> GSMKGSRIELGDVTPHNIKQLKRLNQVIFPVSYNDKFYKDVLEVGELAKLAYFNDI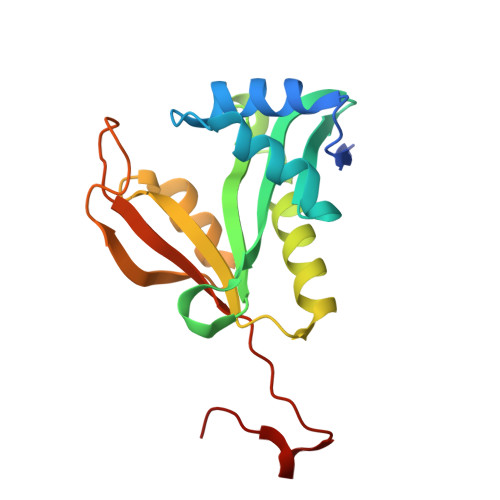AVGAVCCRVDHSQNQKRLYIMTLGCLAPYRRLGIGTKMLNHVLNICEKDGTFDNIYLHVQISNESAIDFYRKFGFEIIETKKNYYKRIEPADAHVLQKNLKVPSGQNADVQKTDN Self-labeling protein tags such as HaloTag are powerful tools that can label fusion proteins with synthetic fluorophores for use in fluorescence microscopy. Here we introduce HaloTag variants with either increased or decreased brightness and fluorescence lifetime compared with HaloTag7 when labeled with rhodamines. To engineer the binding site, ten amino acids on helices 6–8 in close proximity to TMR were chosen for randomization by site-saturation mutagenesis. The changes in spectroscopic properties result from single or double point mutations in the direct vicinity of the bound fluorophore.

The brightest variant, the double mutant HaloTag9 (HaloTag7-Q165H-P174R, ΔI = 19.9 ± 0.5%), as well as the dimmer variants HaloTag10 (HaloTag7-Q165W, ΔI = −52.9 ± 1.2%) and HaloTag11 (HaloTag7-M175W, ΔI = −44.8 ± 0.8%) were chosen for characterization with a panel of 46 different fluorophores and analysis of their photophysical properties. HaloTag9 increased the fluorescence intensity of 16 fluorophores, including rhodamines based on the popular SiR, carbopyronine (CPY) and TMR scaffolds. HaloTag9 showed altered electrostatic surface potential, as well as changes in dihedral angles and rotational energy barriers of the bound TMR compared with HaloTag7, explaining changes in extinction coefficient and quantum yield. On the other hand, the mechanisms behind the increase in fluorescence lifetime observed for HaloTag9 are more complex, involving factors such as changes in electrostatic surface potential or the positioning of the fluorophore on the protein surface. Hence, HaloTag9 showed the longest and HaloTag10 the shortest fluorescence lifetime. All except one fluorophore showed notably higher brightness when bound to HaloTag9 instead of HaloTag7. Photostability measurements showed that the higher the fluorescence lifetime, the more photobleaching occurred, making HaloTag9 the least and HaloTag10 and HaloTag11 the most photostable tags. However, the difference in photostability between HaloTag7 and HaloTag9 is rather small and HaloTag9 is still suitable for stimulated emission depletion (STED) microscopy, which relies on high irradiation intensities. The increased brightness of HaloTag9 relative to HaloTag7 makes it an attractive tool for applications such as fluorescence correlation spectroscopy (FCS) measurements and fluorescence confocal microscopy. Considering that only a limited number of point mutants was screened in this work, we believe that, by targeting other residues for mutagenesis, further increases in fluorescence lifetime of labeled HaloTag9 should be feasible.

>GIGTGFPFDPHYVEVLGERMHYVDVGPRDGTPVLFLHGNPTSSYVWRNIIPHVAPTHRCIAPDLIGMGKSDKPDLGYFFDDHVRFMDAFIEALGLEEVVLVIHDWGSALGFHWAKRNPERVKGIAFMEFIRPIPTWDEWPEFARETFQAFRTTDVGRKLIIDHNVFIEGTLRMGVVRPLTEVEMDHYREPFLNPVDREPLWRFPNELPIAGEPANIVALVEEYMDWLHQSPVPKLLFWGTPGVLIPPAEAARLAKSLPNCKAVDIGPGLNLLQEDNPDLIGSEIARWLSTLEI[2x]GSTs are a multifunctional superfamily of enzymes, distributed in all major kingdoms of living organisms. They are long established to catalyze the conjugation of the tripeptide glutathione with diverse electrophilic and hydrophobic compounds, resulting in their modification to display higher solubility and less toxicity. GSTs that belong to the phi class are dimeric enzymes, comprised of two identical subunits. Residues of the N-terminal domain residues assist the formation of a GSH binding site (G-site), whereas hydrophobic residues of the C-terminal domain form the hydrophobic substrate binding site (H-site).

The structures of sh101 and sh155 enzyme variants were resolved at 1.87 and 2.00 Å resolution and compared to the wild-type AmGSTF enzyme structure that has been recently reported. Sh101 and sh155 were crystallized with two and three molecules in the asymmetric unit, respectively. The sequence between the β2 and β3 strands where the α2 helix is located exhibits significant distortion due to high flexibility. In sh155, high flexibility was observed in the same region in two of the molecules, while in the third one sufficient density was found that enabled the building of the entire loop between β2 and β3. The variants sh101 and sh155 possess 11 and 17 mutations respectively, compared to the wild-type AmGSTF. Among the selected enzymes, sh101 and sh155 exhibited the highest improvement in kcat values (185.9 ± 1.8 min−1 and 197.7 ± 3.2 min−1, respectively), corresponding to an approximately 5-fold improvement, compared to the wild-type AmGSTF enzyme (35.9 ± 1.7 min−1). In particular, the Tm values of sh101 and sh155 enzyme variants were significantly increased by 8.3 and 5.2 °C compared to the parent enzyme AmGSTF. Inspection of the crystal structures of sh101 and sh155 shows that Lys93 can form a new salt bridge with Asp62 of the opposite subunit. However, it was estimated that sh49, sh155 and sh168 exhibited up to 3-fold lower IC50 values than the crop GSTFs. For example, the enzyme variant sh155 could potentially be a promising candidate for the development of a butachlor biosensor, since it combines low IC50 values with high catalytic activity.

>MAPVKVFGPAMSTNVARVTLCLEEVGAEYEVVDIDFKAMEHKSPEHLVRNPFGQIPAFQDGDLLLFESRAIAKYVLRKYKTDEVDLLREGNLKEAAMVDVWTEVDAHTYNPALSPIVYECLINPLMRGLPTNQTVVDESLEKLKKVLEVYEARLSQHKYLAGDFVSFADLNHFPYTFYFMATPHAALFDSYPHVKAWWDRLMARPAVKKIAATMVPPKAHHHHHH[3x]> NIAIERRQGDIA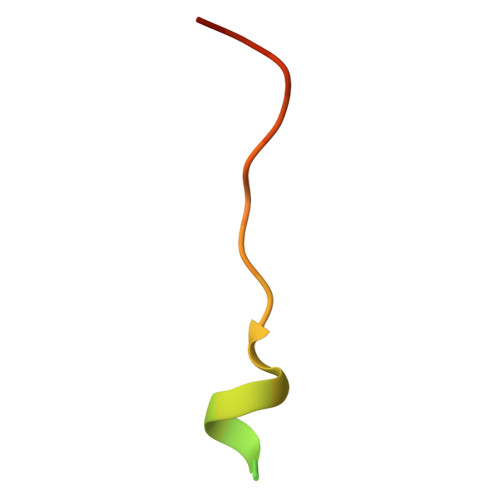ALLIAAGADVNAHAK> MKQKVVSIGDINVANDLPFVLFGGMNVLESRDLAMRICEHYVTVTQKLGIPYVFKASFDKANRSSIHSYRGPGLEEGMKIFQELKQTFGVKIITDVHEPSQAQPVADVVDVIQLPAFLARQTDLVEAMAKTGAVINVKKPQFVSPGQMGNIVDKFKEGGNEKVILCDRGANFGYDNLVVDMLGFSIMKKVSGNSPVIFDVTHALQCRDPFGAASGGRRAQVAELARAGMAVGLAGLFIEAHPDPEHAKCDGPSALPLAKLEPFLKQMKAIDDLVKGFEELDTSK

Here, we introduce an approach to reduce sample waste in SFX experiments at the EuXFEL. It is based on the generation of sub-nL crystal suspension droplets embedded in an immiscible oil, allowing injection with a traditional GDVN. We demonstrate droplet generation of 3-deoxy-D-manno-octulosonate 8-phosphate synthase (KDO8PS) crystal suspensions with a microfluidic droplet generator and show that the droplet generation frequency can be controlled by the flow rates of the aqueous and oil streams. The determined structure revealed new detail in a previously undefined loop region of KDO8PS, a potential target for antibiotic studies.

A room temperature structure of KDO8PS was determined from microcrystals delivered with the segmented flow generator. The SFX structure of KDO8PS was solved based on all collected data where droplet formation was confirmed via the in-line droplet detector. The mean of unit cell constant distributions were calculated to be a = b = c = 118.4 Å and α = β = γ = 90° by cell_explorer, part of the CrystFEL package. Of the 37,000 patterns classified as hits, 16,777 could be indexed and 15,777 patterns were included in the final set of merged reflections (1000 patterns were rejected by partialator during the merging) and used for structure determination. Detected diffraction peaks reached a resolution of 2.8 Å. Our structure represents the apo protein structure at room temperature, wheras the published structures were determined under cryogenic conditions, where cryo-protectant was added. Furthermore, the structures reported by both Radaev et al. and Vainer et al. have a missing, unstructured loop region (residues AA-206 to AA-217), which is believed to be part of the active site of the protein. In the structure presented here, residue CYS-206 showed clear electron density and was therefore included in the model. The electron density revealed differing detail compared to previously-reported KDO8PS structures determined at cryogenic temperatures, such as the CYS-206 residue and a different loop conformation in the residue range 246–251.>MIEEVVAEMIDILAESSKKSIEELARAADNKTTEKAVAEAIEEIARLATAAIQLIEALAKNLASEEFMARAISAIA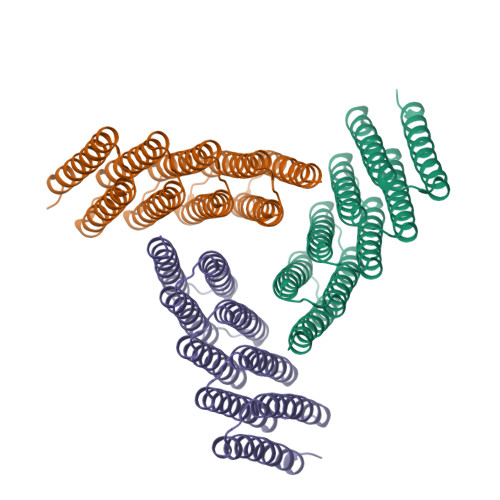ELAKKAIEAIYRLADNHTTDTFMARAIAAIANLAVTAILAIAALASNHTTEEFMARAISAIAELAKKAIEAIYRLADNHTTDKFMAAAIEAIALLATLAILAIALLASNHTTEEFMAKAISAIAELAKKAIEAIYRLADNHTSPTYIEKAIEAIEKIARKAIKAIEMLAKNITTEEYKEKAKSAIDEIREKAKEAIKRLEDNRTLEHHHHHH[3x]>MALINENFLKLKAGYLFPEIARRVKAFTEGNPEAAQRLIRCGIGDVTEALPEAVRYAMHEAVDELGNRSTFKGYGPEQGYDFLRNAIADNDYKARGLPIEADEIFISDGSKCDTGNILDIFGQGNTIAITDPVYPVYVDTNVMIGNTGEADENGAYAGLVYLKCTPENGFVPDIPQEKADLIYLCYPNNPTGAVATRPQLEAWVKYARENGSVLLYDAAYEAFIQDPTIPHSIFEIEGARDCAIEFRSFSKNGGFTGVRCAYVVIPKSLMGRKKNGEAQALHPLWSRRHSTKFNGASYIVQKGAEALYTDEGKSQTKALIEHYMGNAALLVEACKNAGLSVFGGVNAPYVWVGCPAGLTSWQMFDKMLNEANVVITPGSGFGSAGE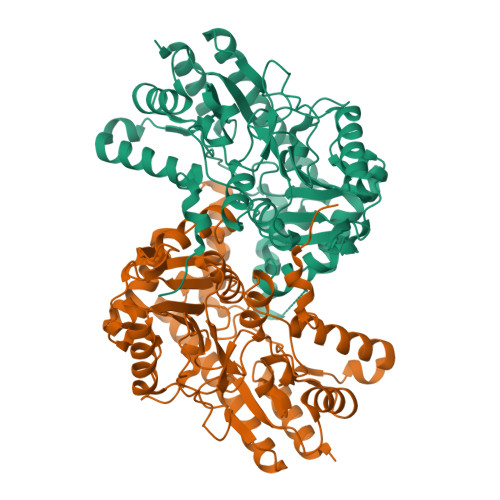GYFRISAFNSRANVEEVCRRIAALK[2x]N-hexanoyl-L-homocysteine | C10 H19 N O3 S | 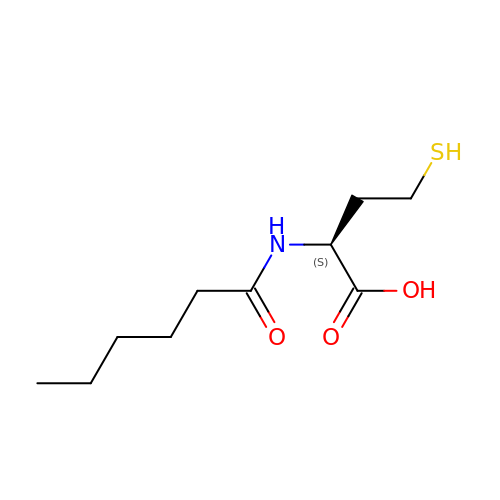HAUWXQBEWNVHPD-QMMMGPOBSA-N>MELPAPVKAIEKQGITIIKTFDAPGGMKGYLGKYQDMGVTIYLTPDGKHAISGYMYNEKGENLS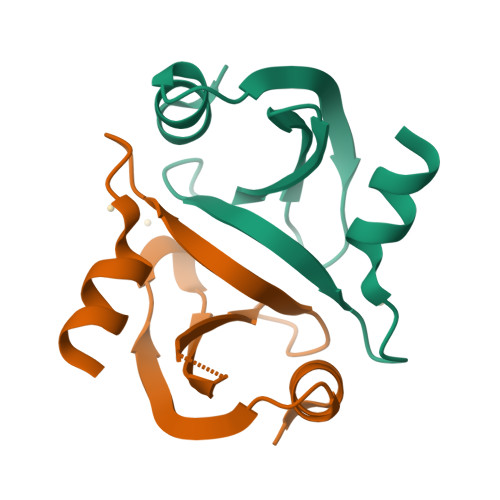NTLIEKEI[2x]3-[4-(5-chloropyridin-3-yl)-2-[(2S)-1-methoxypropan-2-yl]-3-{(1R)-1-[(1r,4R)-4-methylcyclohexyl]ethyl}-3H-imidazo[4,5-c]pyridin-6-yl]-1,2,4-oxadiazol-5(4H)-one 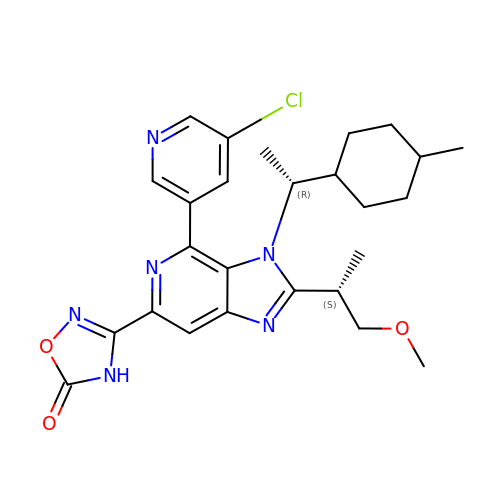| C26 H31 Cl N6 O3 | BOHJWRUCGNOBMS-QBPKDAKJSA-N>MREESWEDHDTIQLTAQRKYLAEVQALETLLTRELSVFLTEPGSKKTNIINRITGKTYALPSTELLRLYEHLEQCRKQGALMYFLERQGTYSGLMLDYDLKLNTNAVPPLEPPALSRLCHRIFVHIKNSSVLPEGSHKIHFFFTLKPEVVQGKYGFHVLIPGLKLAASTKKSIIGSLQHDATVQKILHEQGVTNPESCLDPHSASVPSLLYGSSKLNHKPYQLKTGFELVFDSSDPDYIPIHQIKNLESYNLVSELSLTNEQGSLVRPVYCAADIAAEKEEEIPTEDHSLSILMLHDPEARYLHKILNLLPPEYYVEYPLWSNVVFALANTSANYRPLAEWFSQKCPEKWNTGGKEKLEKLWNDASHHTEKKITKRSIMYWAHKHAPQQYKEIVEQGYFSILAEYVYSYNGMLEHYMIAKVIYAMMGNKFVVDVDSNGKYVWFEFVLPGQPMNQGEIWKWRKEVNPDELHIYISENFSRVMDRITEHIKYHLSQPHESNILNYYKKLLKAFERSKSKIFNDSFKKGVIRQAEFLFRQRSFIQTLDTNPHLLGVGNGVLSIETIPAKLINHFHEHPIHQYTHICYVPFNPENPWTKLLLNALQDIIPELDARLWIMF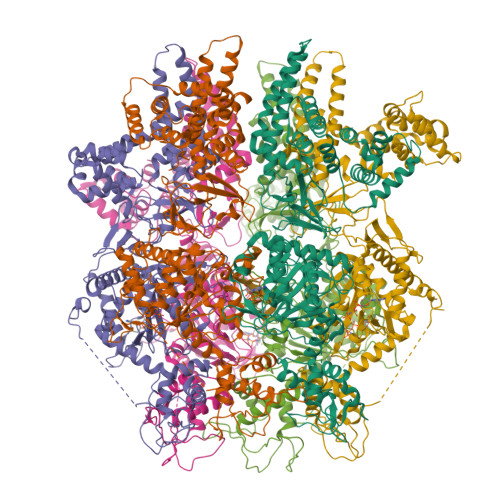YLSTAIFRGLKEALMLLWLGGGCNGKTFLMRLVAMVLGDHYASKLNISLLTSCRETAEKPNSAFMRLKGRGYGYFEETNKSEVLNTSRLKEMVNPGDVTARELNQKQESFQMTATMVAASNYNFIIDTTDHGTWRRLRHYRSKVKFCHNPDPSNPYEKKEDPRFIHEYIMDPDCQNAFFSILVYFWEKLQKEYNGQIKKVFCPTIESETEAYRKSQDTLHRFITERVVESPSAETVYNLSEVVTAYAEWYNTNINVKRHIALELSQELENSVLEKYLQWSPNKTRILKGCRILHKFETLQPGESYIGVSTAGTLLNTPICEPKNKWWEWSPNPSAPPEKEASAPTP[6x]Here, we demonstrate that reduced form of damavaricin C as a vital precursor is finally transformed into MDB-contained mature streptovaricins (streptovaricin C and streptovaricin B or J) by cytochrome P450 enzyme StvP2 after sequential methylation and acetylation. As a result, a component whose retention time, UV/Vis (ultraviolet–visible) spectrum and m/z value are well consistent with 1 was produced (yield > 98%) giving a direct evidence for the function of StvP2 to catalyze MDB formation in mature streptovaricins. To enhance our understanding of MDB formation by StvP2, we solved the X-ray crystal structure of StvP2 at 1.35 Å resolution and the StvP2 in complex with substrate 2 at 2.3 Å resolution, respectively. The overall crystal structures of substrate-free and substrate-bound StvP2 adopts a typical P450 fold, consisted of twelve α-helices (A–L) and two β-sheets (1–2), with a heme as the core cofactor.

To our knowledge, the StvP2 crystal structure in complex with substrate 2 elucidated in this study is the first mechanistic characterization of a cytochrome P450 enzyme catalyzing MDB formation. The high resolution and clear electron density of substrate 2 revealed its high occupancy in the crystal, which also facilitated greatly in substrate 2 molecule model building. The substrate molecule is almost perpendicular to the heme plane in the active pocket. There are multiple interactions between the substrate and the residues of the StvP2. The NH2 group of the amide in Asn69 is hydrogen bonded to the carbonyl O atom of the amide bond in the substrate. Both of the NH of indole ring in Trp74 and the carbonyl O atom in Leu388 are hydrogen bonded to a water molecule, and this water molecule is further bond to the OH group at C21 of the substrate. In addition, the NH2 group and the O atom of carbonyl in Ile390 are bond to the H atom of hydroxyl at C-23 and C-27, respectively. The methoxy group at C-6 in the substrate is pointed toward the iron center of the heme, which is essential to the monooxygenation by P450 enzyme. Moreover, a distinctive catalytic triad (Asp89-His92-Arg72)27,28 observed in the BC loop is considered as the crucial catalytic sites responsible for the important keto-enol tautomerization for further MDB formation, which is never reported so far in this type of reactions and P450 enzymes to the best of our knowledge. Specifically, the carboxyl group of Asp89 is hydrogen bonded to the N-2 atom of imidazole group in His92, and meanwhile, the N-4 atom of imidazole group in His92 is hydrogen bonded to the O atom of the water molecule, which further forms a bifurcated hydrogen bond with the hydroxyl group at the C-1 of the substrate and the imine group of the guanidyl in Arg72, respectively.

>MTETPATPTGLPTARAAGCPFDPPPGLAALRDRAPLTRMEFPNGHVGWLATGHAVVRAVLADPRFSHRNDRRHWPLADIGRGFPPLPGDMLHIDPPDHTRYRKLLAGKFTMRRMRRLTGSAQEIVAGKLDAMERHGGPLDLLEFFARPVPTLMVCALLGVPLQDRATFHPPVRGTDDAAAVEADVAAYVEMTYADMQEYFRKLVAAKRAAPADDLLSDLTTSDLTEDELVGLCAVMMHAGVDSTSNMLALGTWALLERPDQLAALRERPDLADRAVEELMRYMSVVHTGSRAALEDVELAGEVVRAGESVAFSVQAANRDPARFADPDTLDIRRGAVGHLGFGYGVHQCLGMQLARVEMRVAFPALFARFPALRLAVPAGDVPMRDDLVIPYGVHRLPVTW[2x]>IFAEDV[2x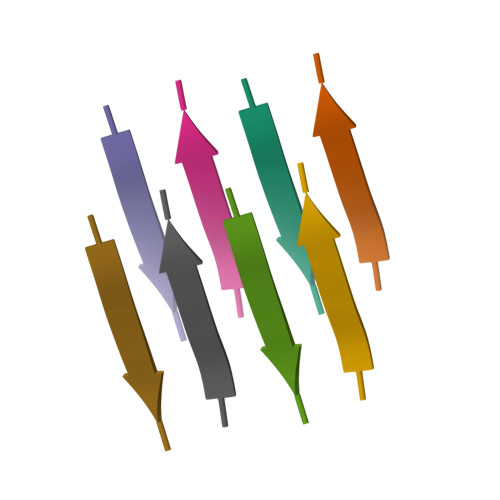]> MGWKTNKY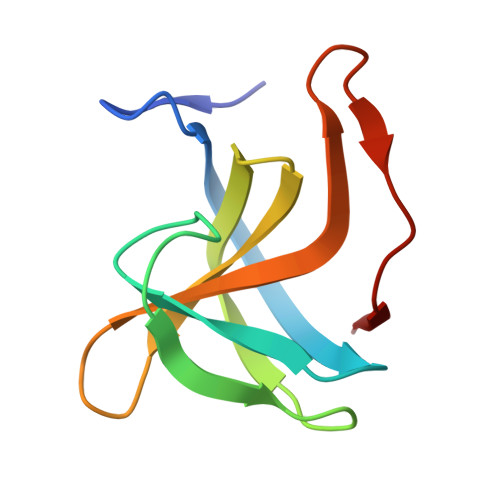GTLYKSESASFTPNTDIITRTTGPFRSMPQSGVLKAGQTIHYDEVMKQDGHVWVGYTGNSGQRIYLPVRTWNKSTNTLGVLWGTIK>[2x]MHRTSNGSHATGGNLPDVASHYPVAYEQTLDGTVGFVIDEM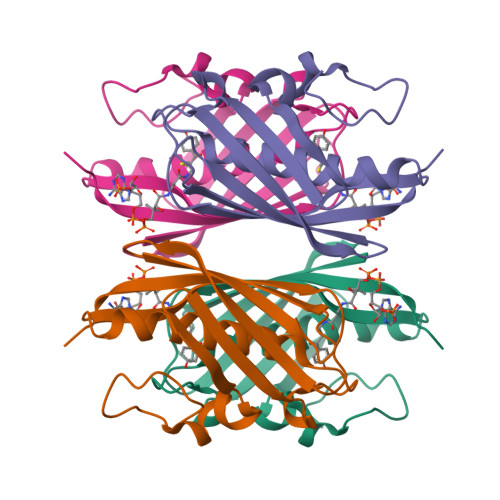TPERATASVEVTDTLRQRWGLVHGGAYCALAQMLATEATVAVVHEKGMMAVGQSNHTSFFRPVKEGHVRAEAVRIHAGSTTWFWDVSLRDDAGRLCAVSSMSIAVRPRRD> SMQRTVAHQITLLECVGKGRYGEVWRGSWQGENVAVKIFSSRDEKSWFRETELYNTVMLRHENILGFIA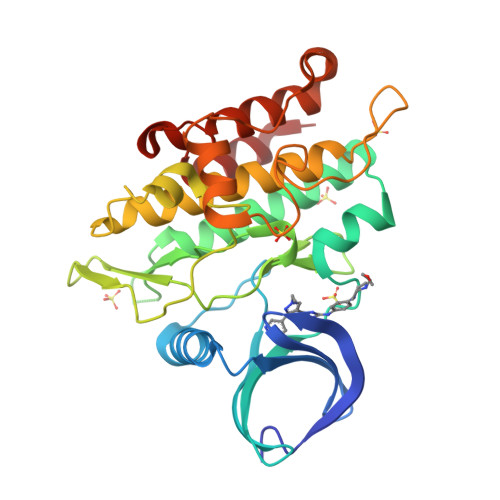SDMTSRHSSTQLWLITHYHEMGSLYDYLQLTTLDTVSCLRIVLSIASGLAHLHIEIFGTQGKPAIAHRDLKSKNILVKKNGQCCIADLGLAVMHSQSTNQLDVGNNPRVGTKRYMAPEVLDETIQVDCFDSYKRVDIWAFGLVLWEVARRMVSNGIVEDYKPPFYDVVPNDPSFEDMRKVVCVDQQRPNIPNRWFSDPTLTSLAKLMKECWYQNPSARLTALRIKKTLTKID> AQSVPYGISQIKAPALHSQGYTGSNVKVAVIDSGIDSSHPDLNVRGGASFVPSETNPYQDGSSHGTHVAGTIAALNNSIGVLGVAPSASLYAVKVLDSTGSGQYSWIINGIEWAISNNMDVINMSLGGPTGSTALKTVVDKAVSSGIVVAAAAGNEGSSGSTSTVGYPAK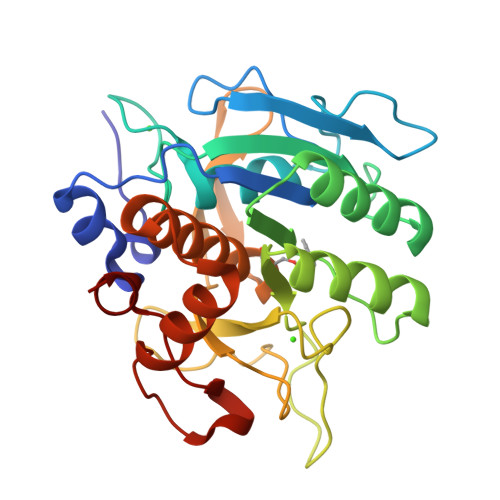YPSTIAVGAVNSSNQRASFSSVGSELDVMAPGVSIQSTLPGGTYGAYNGTSMATPHVAGAAALILSKHPTWTNAQVRDRLESTATYLGNSFYYGKGLINVQAAAQ> MFKAQATFSRYSAAVSLLLLFSGAAQAAPQSITTLPLQPDGENRWRLPAGEYQGQFTIEQPMQLRCEPGAVIQSQGQGSSLLISAPDVLVEGCTLYEWGSDLTAMDSAVFILPAAERAQISNNRMRGPGFGVFVDGTRDVQVIGNEIDGDAGVRSQDRGNGIHLFAVSGARVLHNHVRNARDGIYIDTSNGNHLEGNVIEDVRYGVHYMFANENSLIDNVTRRTRTGYALMQSRKLTVTGNRSEQDQNYGILMNYITYSTITGNFVSDVQRGDTGGDSMISGGEGKALFIYNSLFNTIENNHFEKSSLGIHLTAGSEDNRISGNAFVGNQQQVKYVASRTQEWSVDGRGNYWSDYLGWDRNNDGLGDIAYEPNDNVDRLLWLYPQVRLLMNSPSIEVLRWVQRAFPVIKSPGVQDSHPLMKLPTEKLLTEKQEPTS;>MNAVEIQGVSQRYGSMTVLHDLNLNLGEGEVLGLFGHNGAGKTTSMKLILGLLSPSEGQVKVLGRAPNDPQVRRQLGYLPENVTFYPQLSGRETLRHFARLKGAALTQVDELLEQVGLAHAADRRVKTYSKGMRQRLGLAQALLGEPRLLLLDEPTVGLDPIATQDLYLLIDRLRQRGTSIILCSHVLPGVEAHINRAAILAKGCLQAVGSLSQLRAEAGLPVRIRASGISERDSWLQRWTDAGHSARGLSESSIEVVAVNGHKLVLLRQLLGEGEPEDIEIHQPSLEDLYRYYMERAGDVRAQEGRL[2x];>MNQVWNIARKELSDGLRNRWLLAISLLFAVLAVGIAWLGAAASGQLGFTSIPATIASLASLATFLMPLIALLLAYDAIVGEDEGGTLMLLLTYPLGRGQILLGKFVGHGLILALAVLIGFGCAALAIALLVEGVELGMLFWAFGRFMISSTLLGWVFLAFAYVLSGKVNEKSSAAGLALGVWFLFVLVFDLVLLALLVLSEGKFNPELLPWLLLLNPTDIYRLINLSGFEGSGSAMGVLSLGADLPVPAAVLWLCLLAWIGVSLLLAYAIFRRRLT[2x];> MNALHRIGAGTLLA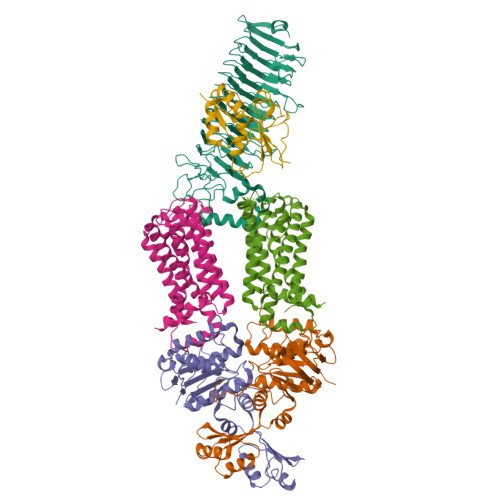VLLAFGLTGCGEKEEVQQSLEPVAFHDSDECHVCGMIITDFPGPKGQAVEKRGVKKFCSTAEMLGWWLQPENRLLDAKLYVHDMGRSVWEKPDDGHLIDATSAYYVVGTSLKGAMGASLASFAEEQDAKALAGMHGGRVLRFEEIDQALLQEAASMQHGGMHDHAPNGAHNAHAGH> MNFSLEGRNIVVMGVANKRSIAWGIARSLHEAGARLIFTYAGERLEKSVHELAGTLDRNDSIILPCDVTNDAEIETCFASIKEQVGVIHGIAHCIAFANKEELVGEYLNTNRDGFLLAHNISSYSLTAVVKAARPMMTEGGSIVTLTYLGGELVMPNYNVMGVAKASLDASVKYLAADLGKENIRVNSISAGPIRTLSAKGISDFNSILKDIEERAPLRRTTTPEEVGDTAAFLFSDMSRGITGEN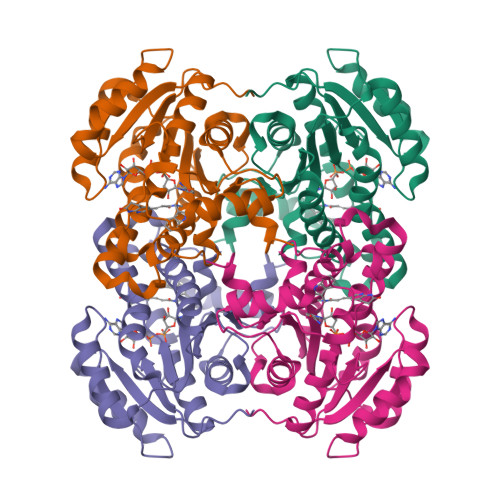LHVDSGFHITARLEHHHHHH> AMADYDTYVSNVQINNLSYGVYTSGGKETQFFCIGLKHGSEAISINAMCKVDVYGNHKQGFDNMLNTAKYYYTTGGDVRIYYKENVWRDPDFKSAFSSRELIAITTCSSSSY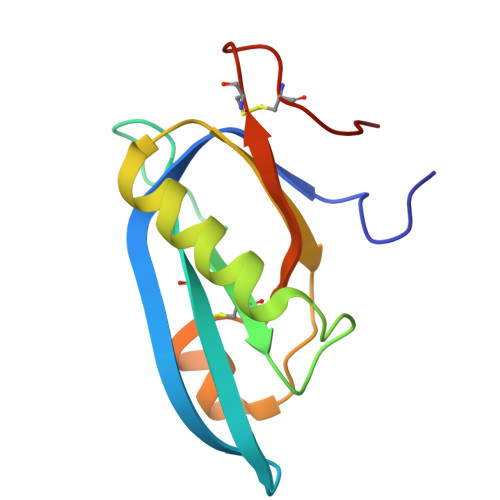CMGPTVTN> GAMGWDGLWDPTLPMIPSANIPGDPIAVVNQVLGISATSAQVTANMGRKFLEQLGILQPTDTGITNAPAGSAQGRIPRVYGRQASEYVIRRG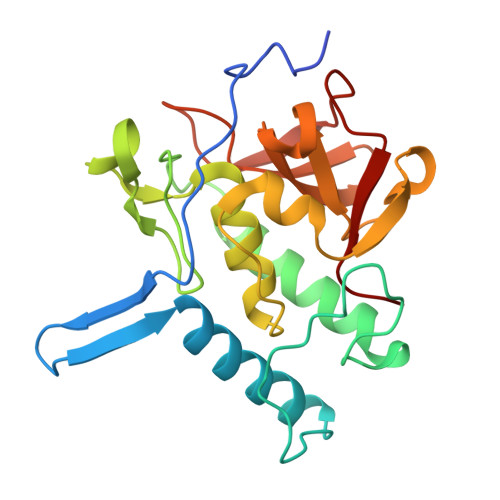MSQIGVPYSWGGGNAAGPSKGIDSGAGTVGFDCSGLVLYSFAGVGIKLPHYSGSQYNLGRKIPSSQMRRGDVIFYGPNGSQHVTIYLGNGQMLEAPDVGLKVRVAPVRTAGMTPYVVRYIEY4-bromo-N-{(2S)-1-[1-(3-fluorophenyl)-4-oxo-1,3,8-triazaspiro[4.5]decan-8-yl]propan-2-yl}benzamide 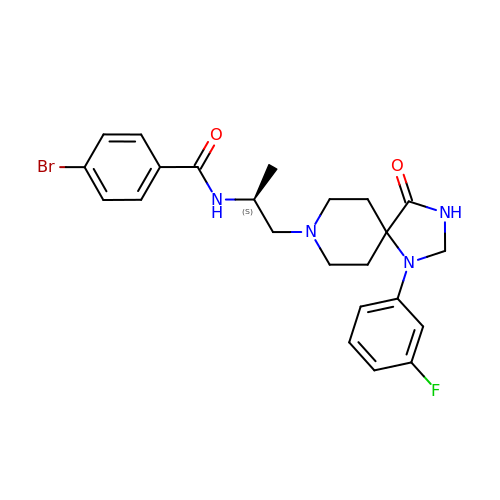| C23 H26 Br F N4 O2 | RFKXAYJUFUZBMA-INIZCTEOSA-N>[2x]MELIRIAMKKDLENDNSLMNKWATVAGLKNPNPLYDFLNHDGKTFNEFSSIVNIVKSQYPDREYELMKDYCLNLDVKTKAARSALEYADANMFFEIEDVLIDSMISCSNMKSKEYGKVYKIHRELSNSVITEFEAVKRLGKLNIKTPEMNSFSRLLLLYHYLSTGNFSPMAQLIKQIDLSEISENMYIRNTYQTRVHVLMSNIKLNENSLEECREYSKKALESTNILRFQVFSYLTIGNSLLFSNYELAQENFLKGLSISVQNENYNMIFQQALCFLNNVWRKENKWINFESDSIMDLQEQAHCFINFNENSKAKEVLDKLDLLVHNDNELAMHYYLKGRLEQNKACFYSSIEYFKKSNDKFLIRLPLLELQKMGENQKLLELLLLLEYA

The arbitrium system comprises three phage genes: (1) AimP, encoding the peptide that is processed into a 6 aa signaling peptide extracellularly, (2) AimR, encoding the intracellular receptor of AimP that is predicted to be structurally similar to RRNPP regulators, and (3) AimX, encoding a putative long non-coding DNA that functions as the negative regulator of lysogeny. As a transcription factor, AimR dimer induces expression of AimX, which promotes lytic cycle. The concentration of AimP will eventually reach the point that its uptake by newly infected bacteria will be high enough to bind AimR and abolish transcriptional activation of AimX, thereby shifting the phage into lysogenic cycle. As predicted from its similarity with RRNPP proteins, the structure of AimR is characterized by two domains, i.e., the N-terminal HTH DNA-binding domain (residues 1–73) and the C-terminal TPR domain (residues 79–386), which are connected by a short linker (residues 74–78).

Due to the high flexibility of N-terminus, the electron density of the apo AimR DBD was weak, which made it challenging to build the structure of residues 1–55. After a strenuous effort, the structure of full-length apo AimR was solved at 2.63 Å resolution using single-wavelength anomalous diffraction method. The final structure of apo AimR contained two molecules in the asymmetric unit spanning residues 1–386 and a C-terminal His-tag. The two protomers within the asymmetric unit are nearly identical, with an average root mean square deviation (RMSD) of 0.159 Å. A notable feature of AimR structure is that it comprises a total of 24 helical secondary structures, including 22 α-helices and two 310-helices. While the first five helices form the DNA binding domain, the remaining α-helices are grouped into eight TPR motifs and a C-terminal capping helix. AimR and AimR-AimP are homodimers and the dimerization is mediated by the C-terminal capping helix, with an approximate solvent-accessible surface of 810 Å2. The residues L380, L383, L384 and L386 contribute to dimerization by engaging in van der Waals interactions with matching residues from the other subunit. The first three α helices in N-terminal DNA-binding domain of apo AimR show a high degree of flexibility. To conclude, we would like to propose an amended mechanistic model of arbitrium system in SPbeta phages, which takes into consideration all three relevant studies (Dou et al., 2018; Wang et al., 2018, and the present study): in the absence of AimP hexapeptide GMPRGA, AimR possesses a highly flexible N-terminal DNA-binding domain.>SDTTIVTVDHKDFDRTEKYLAEHF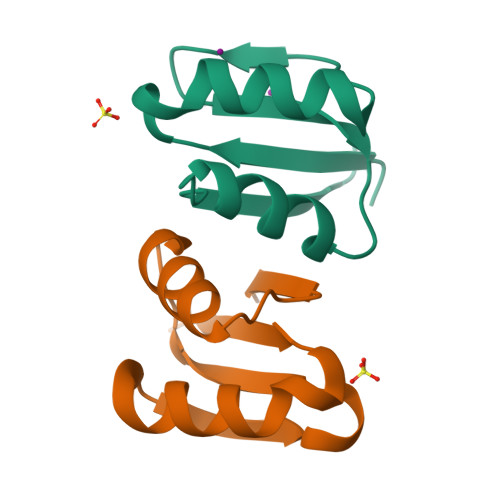QLQNVDKADGHLMINAQKNYQVILKALSELDIYPKYIETRKS[4x]>[8x]GPEPDMISVFIGTWNMGSVPPPKNVTSWFTSKGLGKTLDEVTVTIPHDIYVFGTQENSVGDREWLDLLRGGLKELT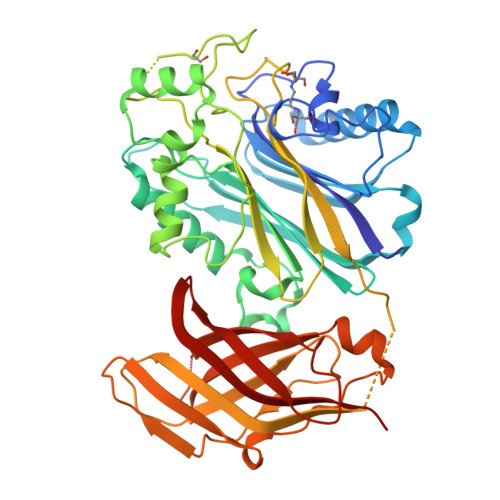DLDYRPIAMQSLWNIKVAVLVKPEHENRISHVSTSSVKTGIANTLGNKGAVGVSFMFNGTSFGFVNCHLTSGNEKTARRNQNYLDILRLLSLGDRQLNAFDISLRFTHLFWFGALNYRLDMDIQEILNYISRKEFEPLLRVDQLNLEREKHKVFLRFSEEEISFPPTYRYERGSRDTYAWHKQKPTGVRTNVPSWCDRILWKSYPETHIICNSYGCTDDIVTSDHSPVFGTFEVGVTSQFISKKGLSKTSDQAYIEFESIEAIVKTASRTKFFIEFYSTCLEEYKKSFENDAQSSDNINFLKVQWSSRQLPTLKPILADIEYLQDQHLLLTVKSMDGYESYGECVVALKSMIGSTAQQFLTFLSHRGEETGNIRGSMKVRVPTER(5S)-2-(methylamino)-5-[(1R)-1-(4-methyl-1H-indol-3-yl)ethyl]-1,3-oxazol-4-one | C15 H17 N3 O2 | 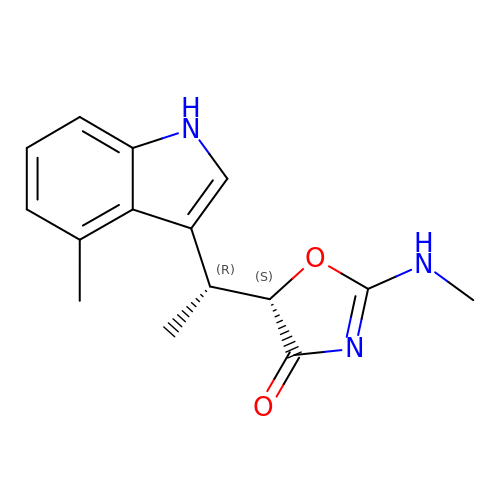SAVVFPXZFDVWPD-RNCFNFMXSA-N>SDKIIHLTDDSFDTDVLKADGAILVDFWAEWCGPCKMIAPILDEIADEYQGKLTVAKLNIDQNPGTAPKYGIRG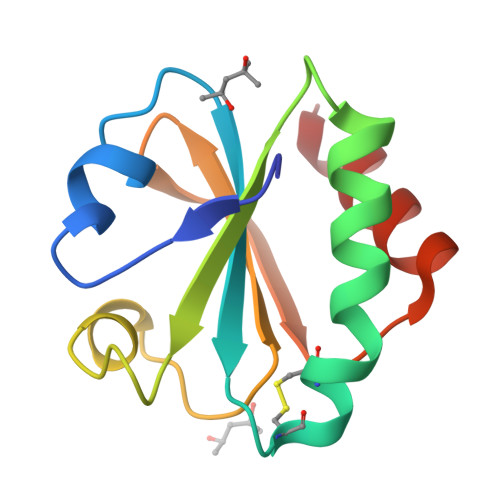IPTLLLFKNGDVAATKVGALSKGQLKEFLDANLA[2x]> MGAQVSTQKTGAHETGLNASGNSIIHYTNINYYKDAASNSANRQDFTQDPGKFTEPVKDI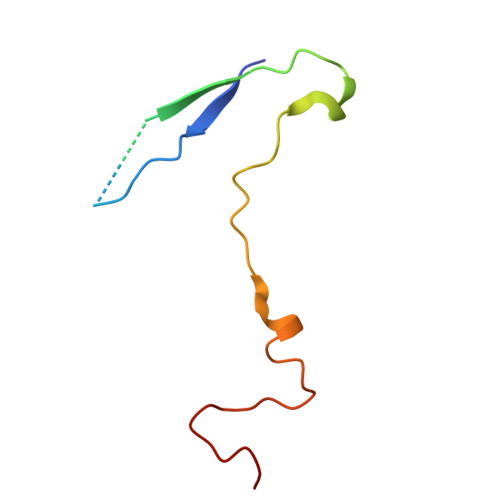MIKSLPALN N,N'-{[(2-{[(2,3-dihydroxyphenyl)carbonyl]amino}ethyl)imino]diethane-2,1-diyl}bis(1-hydroxy-6-oxo-1,6-dihydropyridine-2-carboxamide) 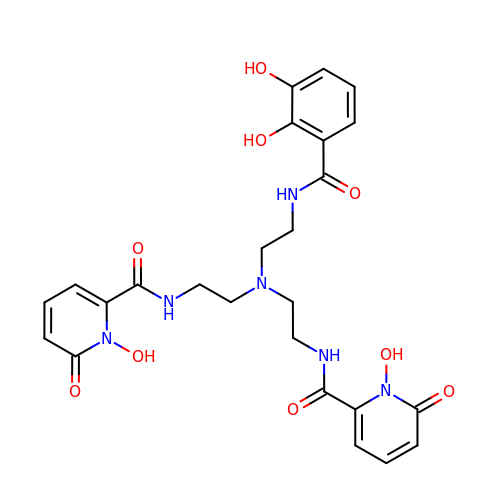| C25 H28 N6 O9 | UPWYYPIMZVCQNS-UHFFFAOYSA-N> MKSNDMNITVELTFFEPYRLVEWFDWDARKKSHSAMRGQAFAQWTWKGKGRTAGKSFITGTLVRSAVIKAVEELLSLNNGKWEGVPCCNGSFQTDESKGKKPSFLRKRHTLQWQANNKNICDKEEACPFCILLGRFDNAGKVHERNKDYDIHFSNFDLDHKQEKNDLRLVDIASGRILNRVDFDTGKAKDYFRTWEADYETYGTYTGRITLRNEHAKKLLLASLGFVDKLCGALCRIEVIKKSESPLPSDTKEQSYTKDDTVEVLSEDHNDELRKQAEVIVEAFKQNDKLEKIRILADAIRTLRLHGEGVIEKDELPDGKEERDKGHHLWDIKVQGTALRTKLKELWQSNKDIGWRKFTEMLGSNLYLIYKKETGGVSTRFRILGDTEYYSKAHDSEGSDLFIPVTPPEGIETKEWIIVGRLKAATPFYFGVQQPSDSIPGKEKKSEDSLVINEHTSFNILLDKENRYRIPRSALRGALRRDLRTAFGSGCNVSLGGQILCNCKVCIEMRRITLKDSVSDFSEPPEIRYRIAKNPGTATVEDGSLFDIEVGPEGLTFPFVLRYRGHKFPEQLSSVIRYWEENDG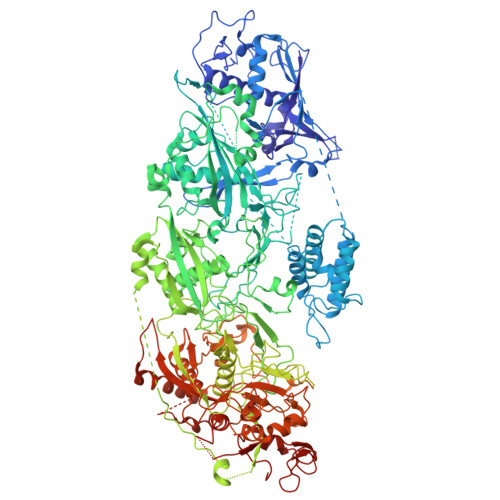KNGMAWLGGLDSTGKGRFALKDIKIFEWDLNQKINEYIKERGMRGKEKELLEMGESSLPDGLIPYKFFEERECLFPYKENLKPQWSEVQYTIEVGSPLLTADTISALTEPGNRDAIAYKKRVYNDGNNAIEPEPRFAVKSETHRGIFRTAVGRRTGDLGKEDHEDCTCDMCIIFGNEHESSKIRFEDLELINGNEFEKLEKHIDHVAIDRFTGGALDKAKFDTYPLAGSPKKPLKLKGRFWIKKGFSGDHKLLITTALSDIRDGLYPLGSKGGVGYGWVAGISIDDNVPDDFKEMINKTEMPLPEEVEESNNGPINNDYVHPGHQSPKQDHKNKNIYYPHYFLDSGSKVYREKDIITHEEFTEELLSGKINCKLETLTPLIIPDTSDENGLKLQGNKPGHKNYKFFNINGELMIPGSELRGMLRTHFEALTKSCFAIFGEDSTLSWRMNADEKDYKIDSNSIRKMESQRNPKYRIPDELQKELRNSGNGLFNRLYTSERRFWSDVSNKFENSIDYKREILRCAGRPKNYKGGIIRQRKDSLMAEELKVHRLPLYDNFDIPDSAYKANDHCRKSATCSTSRGCRERFTCGIKVRDKNRVFLNAANNNRQYLNNIKKSNHDLYLQYLKGEKKIRFNSKVITGSERSPIDVIAELNERGRQTGFIKLSGLNNSNKSQGNTGTTFNSGWDRFELNILLDDLETRPSKSDYPRPRLLFTKDQYEYNITKRCERVFEIDKGNKTGYPVDDQIKKNYEDILDSYDGIKDQEVAERFDTFTRGSKLKVGDLVYFHIDGDNKIDSLIPVRISRKCASKTLGGKLDKALHPCTGLSDGLCPGCHLFGTTDYKGRVKFGFAKYENGPEWLITRGNNPERSLTLGVLESPRPAFSIPDDESEIPGRKFYLHHNGWRIIRQKQLEIRETVQPERNVTTEVMDKGNVFSFDVRFENLREWELGLLLQSLDPGKNIAHKLGKGKPYGFGSVKIKIDSLHTFKINSNNDKIKRVPQSDIREYINKGYQKLIEWSGNNSIQKGNVLPQWHVIPHIDKLYKLLWVPFLNDSKLEPDVRYPVLNEESKGYIEGSDYTYKKLGDKDNLPYKTRVKGLTTPWSPWNPFQVIAEHEEQEVNVTGSRPSVTDKIERDGKMV> ADTYAATRYPVILVHGLAGTDKFANVVDYWYG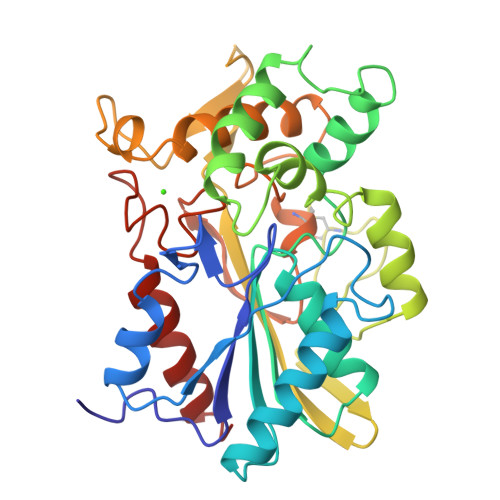IQSDLQSHGAKVYVANLSGFQSDDGPNGRGEQLLAYVKQVLAATGATKVNLIGHSQGGLTSRYVAAVAPQLVASVTTIGTPHRGSEFADFVQDVLKTDPTGLSSTVIAAFVNVFGTLVSSSHNTDQDALAALRTLTTAQTATYNRNFPSAGLGAPGSCQTGAATETVGGSQHLLYSWGGTAIQPTSTVLGVTGATDTSTGTLDVANVTDPSTLALLATGAVMINRASGQNDGLVSRCSSLFGQVISTSYHWNHLDEINQLLGVRGANAEDPVAVIRTHVNRLKLQGV> MAHHHHHHSSGLEVLFQMEQNPQSQLKLLVTRGKEQGYLTYAEVNDHLPEDIVDSDQIEDIIQMINDMGIQVMEEAPDADDLMLAENTADEDAAEAAAQVLSSVESEIGRTTDPVRMYMREMGTVELLTREGEIDIAKRIEDGINQVQCSVAEYPEAITYLLEQYDRVEAEEARLSDLITGFVDPNAEEDLAPTATHVGSELSQEDLDDDEDEDEEDGDDDSADDDNSIDPELAREKFAELRAQYVVTRDTIKAKGRSHATAQEEILKLSEVFKQFRLVPKQFDYLVNSMRVMMDRVRTQERLIMKLCVEQCKMPKKNFITLFTGNETSDTWFNAAIAMNKPWSEKLHDVSEEVHRALQKLQQIEEETGLTIEQVKDINRRMSIGEAKAR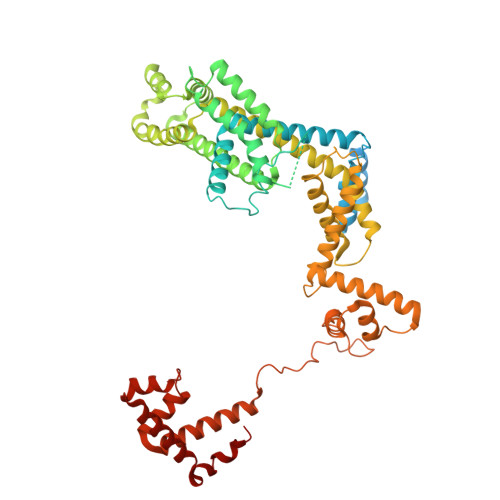RAKKEMVEANLRLVISIAKKYTNRGLQFLDLIQEGNIGLMKAVDKFEYRRGYKFSTYATWWIRQAITRSIADQARTIRIPVHMIETINKLNRISRQMLQEMGREPTPEELAERMLMPEDKIRKVLKIAKEPISMETPIGDDEDSHLGDFIEDTTLELPLDSATTESLRAATHDVLAGLTAREAKVLRMRFGIDMNTDYTLEEVGKQFDVTRERIRQIEAKALRKLRHPSRSEVLRSFLDD> MSTYEGRWKTVKVEIEDGIAFVILNRPEKRNAMSPTLNREMIDVLETLEQDPAAGVLVLTGAGEAWTAGMDLKEYFREVDAGPEILQEKIRREASQWQWKLLRM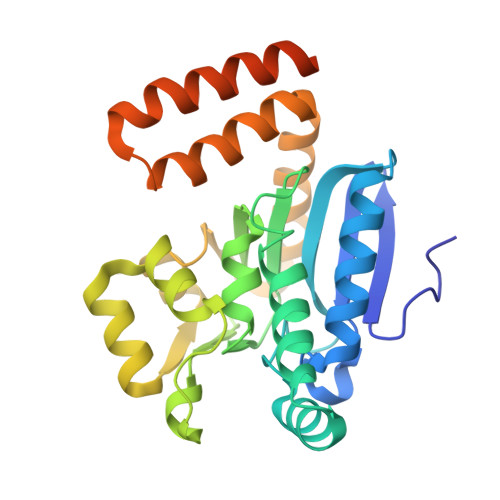YAKPTIAMVNGWCFGGGFSPLVACDLAICADEATFGLSEINWGIPPGNLVSKAMADTVGHRQSLMYIMTGKTFGGQKAAEMGLVNESVPLAQLREVTIELARNLLEKNPVVLRAAKHGFKRCRELTWEQNEDYLYAKLDQSRLLDTEGGREQGMKQFLDDKSIKPGLQAYKR> MDFLTSTLLSGILYDGFKNGVAITTGFLKEKL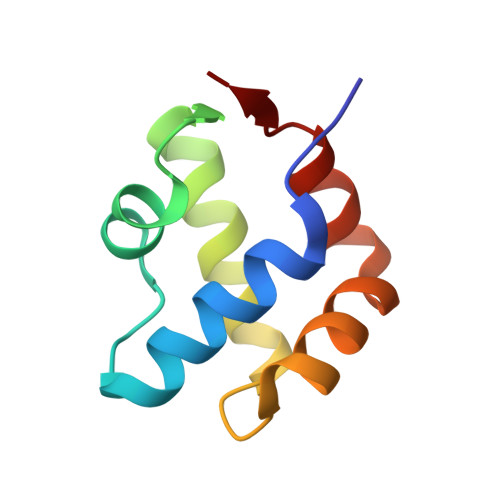HGWIVDDTLLETLAYKVNTLELKDYGEHVIERKLNESSEIQQILKLIQPE>MQSIRCLALAAVALFMAGCSSFTSESATPLARGAQWGLVPLLNYSQAPQAGERAEQILLSVLAEEGVRPRLYPAQPQGDLQLVDDRERQQRALDWARQQKLAYVVTGSVEEWQYKNGLDGEPAVGVSLQVLEPASGRVLWSTSGARAGWSRESLAGAAQKVLRELVGDLRLE[12x];> MANSSAADKHPQARLLNPWALLPVALGVALVLWLTFNSEEVFMPSGDGEPDAVSVNYAELLLQAHPENDALRLTLIDLLVKLGDFEQARHHLARLRGKDRLATPFYEVELDILGALARPEGMDEEQTRRLLERLRKIEHVSLNDAMLERLARHALALDAPDLAARTFAELAGRDPQGRQRWLDEAARWYLASGEPLPAADIQRQLAEAQTEPAKRLAYLRQAFASLLAGERGEQAALLLDERLDALPEDESTLAWLAQGVRAAEGSQRYDLAERFIRRWRELRPEDHEALAADLRLNMAAGRVERAWEVGQELLALRPEDRTLLADLARLGEWTGNGPRALGFWKQLLAGADDPALREHAWRLSLQMFDFDSAIELLAPIGAQRQMTDEELDALVYSHETRGTPEEGEAWLRGYVQRYPKQRLAWQRLQQILEHTQQLQEETGVWARMARHFPLSVKERMQWAETHWNLFDPRQAWKVLAGVDTRAIREPEFWRLRAALAWALEQDDDARAAYERMLALDIRLNSRDEDQLIALYRDSNPKQALQVLIGSWQRSRDPRRLASALQLAENLHDWPALKSLLAEAEGLPEAQGSPYYWVARARLAEQEGHGDVAERLYREALVRFPGENLVRERLLWFYIDRGRRDSLAPLLAQWHGLALRDSTLWLPFASASLLLERNDQALAWFRLYLKSNPNDWLVQAAYADALDASGYQDKALRLRRLLLRRLDREAVRATPDSFATYLRLLAVAQGPLLAQGEARRAWNGEPAMLQLWFEQFLDQLAATNQEPLKDNWLAWARGRGLKIGRNEEIQAALRSQNRAALQRLLERGELDPAQRVEALVRLGHGGEALGEALGALGDGHSRDNREQLRRQAAEILERTPQGLQLGWNKRDFGGLDFKGPTLRAARHLGDDWYADLELGSGRYHGDALDSSLLGSERNARLTLRRELADGFAAATLDGSWRDDEDRHGLGVLRNWRLSSRDELEAGLDWHRETDETGLMRALGMRDSLRLGGRHTLSGRDQLSWSLAHNRFSTRQGDDLGNGEALSLEWAHTLFFDGPAWQLRGGIDYQRNRLENRVPDDLLAAHGGALALDGARSQDLLQDRYGQVYLGSTWRRGFPGALNRSRPQYTWIVDTLAGWQWTEKEFNYGIDLGIGMELLGDDELAFTFGYQSAPQGGGGDAGGTLGVTYSTRFGR

Here, we reveal the architecture of the outer membrane complex PelBC for Pel export, where the essential periplasmic ring of twelve lipoproteins PelC is mounted on top of the nanodisc-embedded β-barrel PelB. Pel is the major constituent of P. aeruginosa pellicles, i.e., films formed at the water-air interface, and it plays a key role at early stages of the biofilm formation at solid surfaces. P. aeruginosa Pel is composed of α−1-4-linked N-acetyl-D-galactosamine residues, which are partially deacetylated in the periplasm, so the Pel exopolysaccharide acquires positive charge along the secretion pathway. The β-barrel of PelB is assumed to form a complex with PelC lipoproteins, a hallmark of the Pel system in Gram-negative bacteria.

Here, we employed cryogenic electron microscopy (cryo-EM) to visualize the structure of the PelBC complex of P. aeruginosa in the lipid-based nanodiscs, reaching a final resolution of 2.5 Å. In agreement with the prediction, the complex is composed of a single PelB barrel built of 16 antiparallel β-strands embedded in the lipid bilayer and a dodecameric ring of PelC lipoproteins mounted at the periplasmic side. At the periplasmic side of PelB, two TPR domains resolved from the residues Gly-803 and the intermediate helix (“stalk”) are located within the PelC ring, being docked at multiple lipoprotein subunits. The interior of the PelB β-barrel is predominantly negatively charged, where the charge is distributed asymmetrically, being largely concentrated on strands 11 to 14. As a major element here, a short α-helix between the strands 7 and 8 (further referred as Plug-I) is bent inwards the central cavity of PelB where it lays perpendicular to the barrel axis. Plug-I is opposed by a glycine-rich loop between the C-terminal β-strands 15 and 16 (Plug-S), and together these two loops occlude the exit tunnel of PelB. However, the exit pore within the resolved PelB structure is occluded by the glycine-rich loop Plug-S with a bottleneck width of 4 Å. However, within the assembled complex those aspartates are buried at the PelB-PelC interface and build multiple contacts with the surface-exposed arginine residues of PelB, such as 905, 944, 1018, 1114, 1122, and 1190, thus playing rather a structural role. The anchor chains of individual PelC subunits are sandwiched between two Trp-149 residues, one from the same PelC, and one from a preceding subunit, a configuration that potentially facilitates docking of the lipoproteins at the membrane interface. A fully resolved lipid molecule was located between the PelC subunits H and I, forming extensive interactions with the lipoproteins and the barrel.> GELGSPTYLEPGIGRHTPYGNQTDYRIFELNKRLQNWTEECDNLWWDAFTTEFFEDD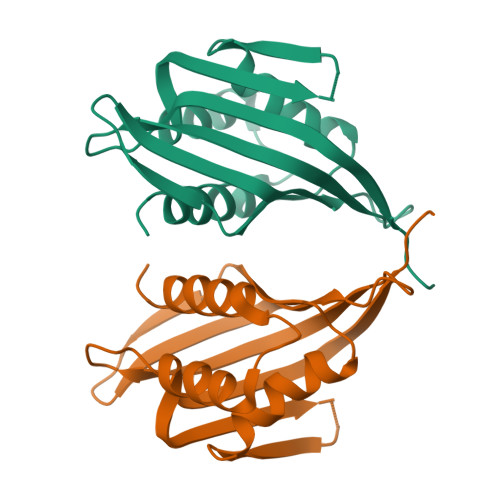AMLTITFCLEDGPKRYTIGRTLIPRYFRSIFEGGATELYYVLKHPKEAFHSNFVSLDCDQGSMVTQHGKPMFTQVCVEGRLYLEFMFDDMMRIKTWHFSIRQHRELIPRSILAMHAQDPQMLDQLSKNITRCGLS>[2x]MASLNTPAPLPTSCNPSDMSHGYVTVKPRVRLHFVELGSGPAVCLCHGFPESWYSWRYQIPALAQAGYRVLAMDMKGYGESSAPPEIEEYCMEVLCKEMVTFLDKLGLSQAVFIGHDWGGMLV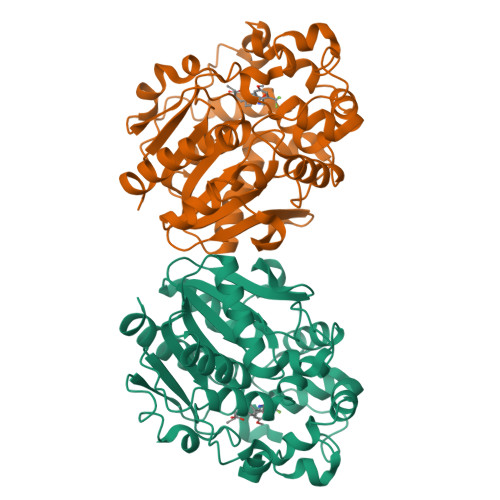WYMALFYPERVRAVASLNTPFIPANPNMSPLESIKANPVFDYQLYFQEPGVAEAELEQNLSRTFKSLFRASDESVLSMHKVCEAGGLFVNSPEEPSLSRMVTEEEIQFYVQQFKKSGFRGPLNWYRNMERNWKWACKSLGRKILIPALMVTAEKDFVLVPQMSQHMEDWIPHLKRGHIEDCGHWTQMDKPTEVNQILIKWLDSDARNPPVVSKMLLEHHHHHH> MSENLKDEILEKYIPKTKKTRSGH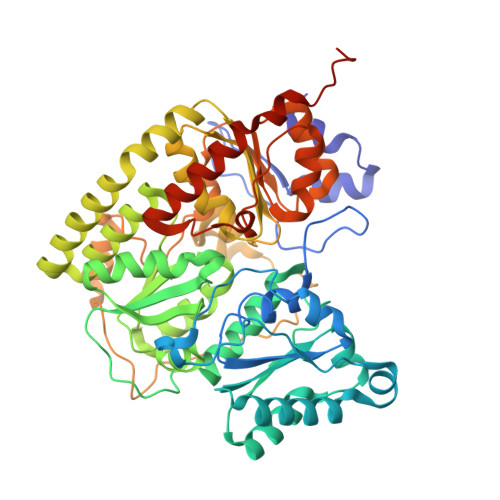IVIKTEETPNPEIVANTRTVPGIITARGCAYAGCKGVVMGPIKDMVHITHGPIGCSFYTWGGRRFKSKPENGTGLNFNEYVFSTDMQESDIVFGGVNKLKDAIHEAYEMFHPAAIGVYATCPVGLIGDDILAVAATASKEIGIPVHAFSCEGYKGVSQSAGHHIANNTVMTDIIGKGNKEQKKYSINVLGEYNIGGDAWEMDRVLEKIGYHVNATLTGDATYEKVQNADKADLNLVQCHRSINYIAEMMETKYGIPWIKCNFIGVDGIVETLRDMAKCFDDPELTKRTEEVIAEEIAAIQDDLDYFKEKLQGKTACLYVGGSRSHTYMNMLKSFGVDSLVAGFEFAHRDDYEGREVIPTIKIDADSKNIPEITVTPDEQKYRVVIPEDKVEELKKAGVPLSSYGGMMKEMHDGTILIDDMNHHDMEVVLEKLKPDMFFAGIKEKFVIQKGGVLSKQLHSYDYNGPYAGFRGVVNFGHELVNGIYTPAWKMITPPWKKASSESKVVVGGEA> MSFINYSSREINCKIVYYGPGLCGKTTNLQYIYNKTAAETKGKLISLSTETDRTLFFDFLPLSLGEIRGFKTRFHLYTVPGQVFYDASRKLILKGVDGVVFVADSQIERMEANMESLENLRINLAEQGYDLNKIPYVIQYNKRDLPN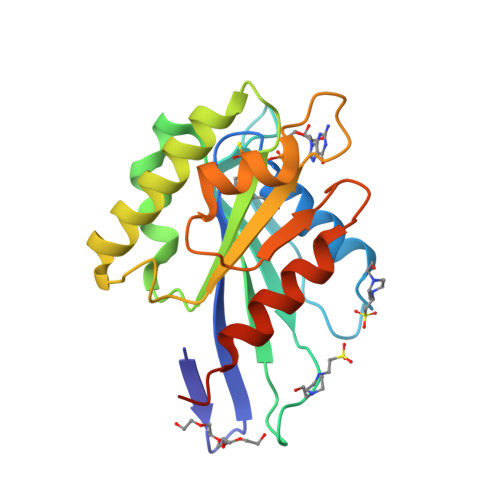AVTVEEMRKALNHRNIPEYQAVAPTGVGVFDTLKAVAKLVLTELKKGGHHHHHH;>GMGTQLVMYEEEFTKINAVCDRLTKDANAKVVFLVDKNGQLISSAGQTQNIDTTSLASLTAGNVAAMGGLAKLIGENEFPNQFHEGAKDSLYMTIVGSRVVLVVIFDNRTSLGLVRLRIKKASDELTKIFESLVKKTDSPGAGSPFAEISDDDIDNLFSE[2x]>[4x]GSHMLTPTLVSLLEVIEPEVLYAGYDSSVPDSTWRIMTTLNMLGGRQVIAAVKWAKAIPGFRNLHLDDQMTLLQYSWMSLMAFALGWRSYRQSSA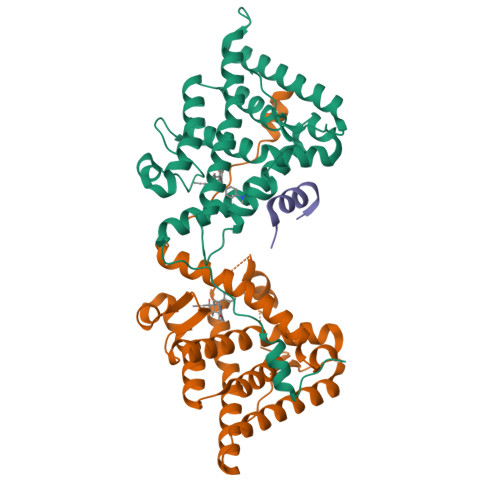NLLCFAPDLIINEQRMTLPDMYDQCKHMLYVSSELHRLQVSYEEYLCMKTLLLLSSVPKDGLKSQALFDAIRMTYIKELGKAIVKREGNSSQNSQRFYQLTKLLDSMHEVVENLLNYCFQTFLDKTMSIEFPEMLAEIITNQIPKYSNGNIKKLLFHQK;>ASNLGLEDIIRKALMGSFD[2x]3',3'-cdUMP | C18 H24 N4 O16 P2 | 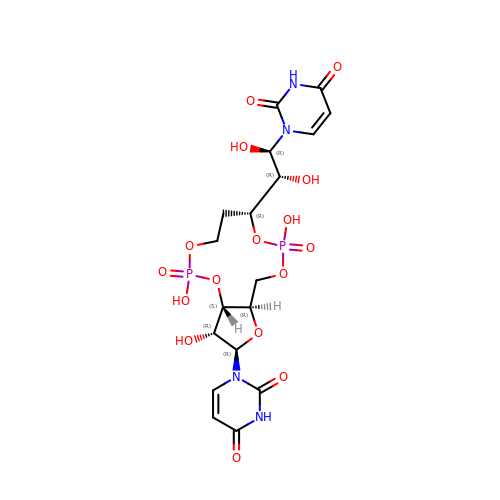SDBXSRQCWCPJQL-WXFFCYTBSA-N>MSKWTYFGPDGENSWSKKYPSCGGLLQSPIDLHSDILQYDASLTPLEFQGYNLSANKQFL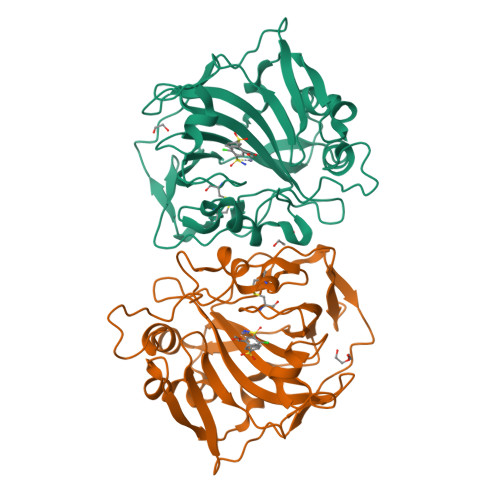LTNNGHSVKLNLPSDMHIQGLQSRYSATQLHLHWGNPNDPHGSEHTVSGQHFAAELHIVHYNSDLYPDASTASNKSEGLAVLAVLIEMGSFNPSYDKIFSHLQHVKYKGQEAFVPGFNIEELLPERTAEYYRYRGSLTTPPCNPTVLWTVFRNPVQISQEQLLALETALYCTHMDDPSPREMINNFRQVQKFDERLVYTSFSQ[4x]>[4x]GSHMSFRDNLKVYIESPESYKNVIYYDDDVVLVRDMFPKSKMHLLLMTRDPHLTHVHPLEIMMKHRSLVEKLVSYVQGDLSGLIFDEARNCLSQQLTNEALANYIKVGFHAG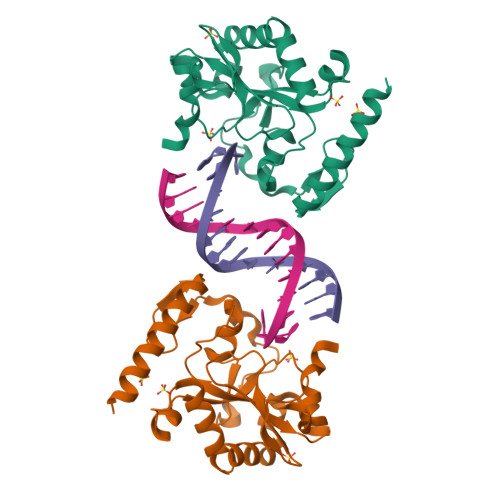PSMNNLHLHIMTLDHVSPSLKNSAHYISFTSPFFVKIDTPTSNLPTRGTLTSLFQEDLKCWRCGETFGRHFTKLKAHLQEEYDDWLDKSVSM> MATLSLTVNSGDPPLGALLAVEHVKDDVSISVEEGKENILHVSENVIFTDVNSILRYLARVATTAGLYGSN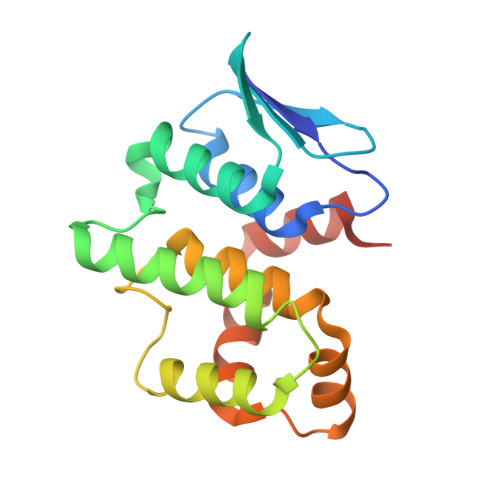LMEHTEIDHWLEFSATKLSSSDSFTSTINELNHSLSLRTYLVGNSLSLADLSVWATLKGNAAWQEQLKQKKAPVHVKRWFGFLEAQQAFQSVGTKWDVSTTKAR TDases are class A flavin-dependent monooxygenases that covalently modify and inactivate the core tetracycline moiety. Here, we investigate Tet(X6), a type 1 TDase first discovered in a Proteus genomospecies, by determining anhydrotetracycline-free and anhydrotetracycline-complexed X-ray crystal structures. Tet(X6) inactivates all classes of tetracyclines demonstrated by in vitro enzyme assays and phenotypic studies in E. coli. Here, we present structural, biochemical, and phenotypic evidence that anhydrotetracycline binds in a substrate-like orientation and competitively inhibits the type 1 TDase Tet(X6) to rescue tetracycline antibiotic activity as a sacrificial substrate.

We determined the X-ray structure of Tet(X6) at 2.2 Å resolution with Rfree/Rwork of 0.22/0.19. This FAD complexed, anhydrotetracycline-free enzyme structure consists of a conserved architecture for type 1 TDases: a characteristic Rossman fold containing an FAD-binding domain, a substrate binding domain, and a C-terminal bridge helix that connects the two domains. The 393 amino acid long polypeptide chain alternates four times between the substrate-binding domain and FAD-binding domain. The FAD cofactor is bound in an “IN” orientation in Tet(X6). Thus far, the FAD conformation in structures of type 1 TDases have only been captured in this “IN” orientation, while structures of type 2 TDases have been solved for both “IN” and “OUT” orientations. The conserved FAD-interacting residues include Pro26, Val27, Gly28, Glu46, Arg47, Thr59, Arg117, Leu139, and Val324. The conserved substrate-binding residues are Gln192, Arg213, Phe224, His234 and Gly236. Met375 of the C-terminal bridge helix also interacts with the bound tetracycline substrate and is conserved among the type 1 TDases.

> MTSSSHHHHHHSSGKLMTLKPANKNMTLLKHKKITIIGAGPVGLTMARLLQQNGVDITVYERDKDQDARIFGGTLDLHRDSGQEAMKRAGLLQTYYDLALPMGVNIVDEKGNILTTKNVRPENRFDNPEINRNDLRTILLNSLQNDTVIWDRKLVTLEPDKEKWILTFEDKSSETADLVIIANGGMSKVRKFVTDTEVEETGTFNIQADIHQPEVNCPGFFQLCNGNRLMAAHQGNLLFANPNNNGALHFGISFKTPDEWKSKTRVDFQDRNSVVDFLLKKFSDWDERYKELIRLTSSFVGLATRIFPLDKSWKSKRPLPITMIGDAAHLMPPFAGQGVNSGLMDALILSDNLTNGKFNSIEEAIENYEQQMFAYGREAQAESIINETEMFSLDFSFQKLMNL>[2x]MAHHHHHHMSLAVEAVKDFLLKLQDDICEALEAEDGQATFVEDKWTREGGGGGRTRVMVDGAVIEKGGVNFSHVYGKGLPMSSTERH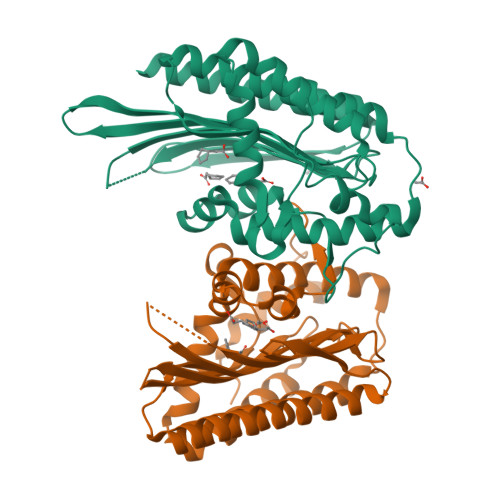PDIAGCNFEAMGVSLVIHPKNPHVPTSHANVRLFVAEREGKEPVWWFGGGFDLTPYYAVEEDCRDFHQVAQDLCKPFGADVYARFKGWCDEYFFIPYRNEARGIGGLFFDDLNEWPFEKCFEFVQAVGKGYMDAYIPIVNRRKNTPYTEQQVEFQEFRRGRYAEFNLVIDRGTKFGLQSGGRTESILISLPPRARWGYNWQPEPGTPEARLTEYFLTKRQWV>SKPFSLPILTLSELTNSRFPVPIDSLFTAQNNVLQVQCQNGRCTLDGELQGTTQLLPTGICAFRGRVTAQINQRDRWHMQLQNLNGTTYDPTDDVPAPLGTPDFKGVVFGMVSQRNVGNDAPGSTRAQQAWVSTYSPQFVPKLGSVNLRISDNDDFQFQPTKFTPVGVNDDDDGHPFRQWELPNYSGELTLNMNLAPPVAPNFPGEQLLFFRSFVPCSGGYNQGIIDCLIPQEWIQHFYQESAPSQSDVALIRYVNPDTGRTLFEAKLHRSGYITVAHS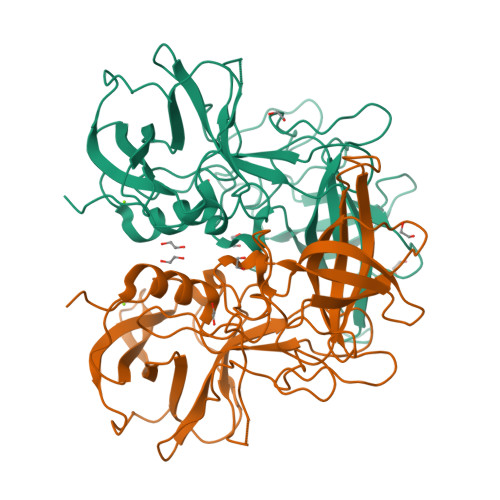GDYPLVVPANGHFRFDSWVNQFYSLAPM[2x]>[2x]MSQ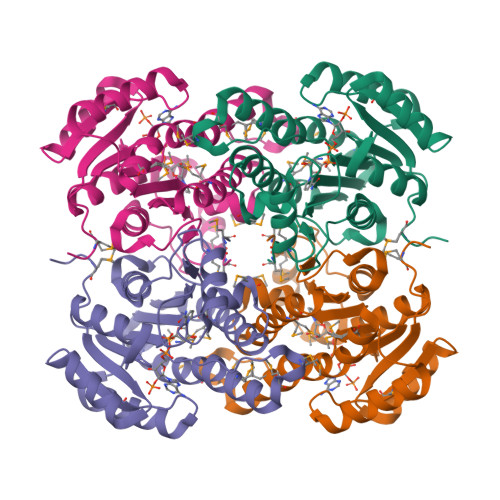FMNLEGKVALVTGASRGIGKAIAELLAERGAKVIGTATSESGAQAISDYLGDNGKGMALNVTNPESIEAVLKAITDEFGGVDILVNNAGITRDNLLMRMKEEEWSDIMETNLTSIFRLSKAVLRGMMKKRQGRIINVGSVVGTMGNAGQANYAAAKAGVIGFTKSMAREVASRGVTVNTVAPGFIETDMTKALNDEQRTATLAQVPAGRLGDPREIASAVAFLASPEAAYITGETLHVNGGMYMI>GSMRNEVQFELFGDYALFTDPLTKIGGEKLSYSVPTYQALKGIAESIYWKPTIVFVIDELRVMKPIQMESKGVRPIEYGGGNTLAHYTYLKDVHYQVKAHFEFNLHRPDLAFDRNEGKHYSILQRSLKAGGRRDIFLGARECQGYVAPCEFGSGDGFYDGQ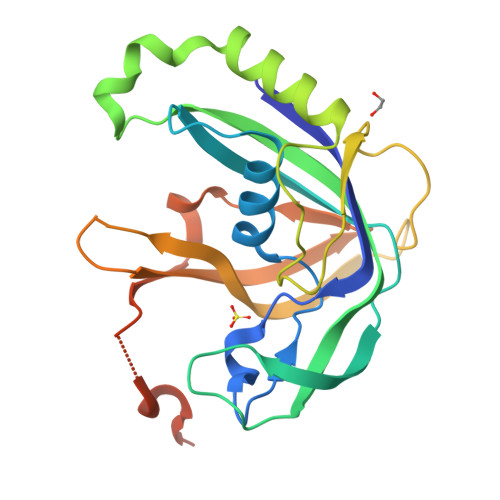GKYHLGTMVHGFNYPDETGQHQLDVRLWSAVMENGYIQFPRPEDCPIVRPVKEMEPKIFNPDNVQSAEQLLHDLGGE[2x]>SNAMTGLFVTLEGPEGAGKSTNRDYLAERLRERGIEVQLTREPGGTPLAERIRELLLAPSDEPMAADTELLLMFAARAQHLAGVIRPALARGAVVLCDRFTDATYAYQGGGRGLPEARIAALESFVQGDLRPDLTLVFDLPVEIGLARAAARGRLDRFEQEDRRFFEAVRQTYLQRAAQAPERYQVLDA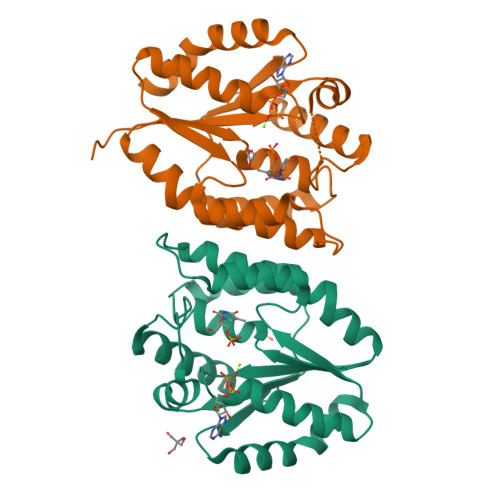GLPLAEVQAGLDRLLPNLLERLNG[2x]> G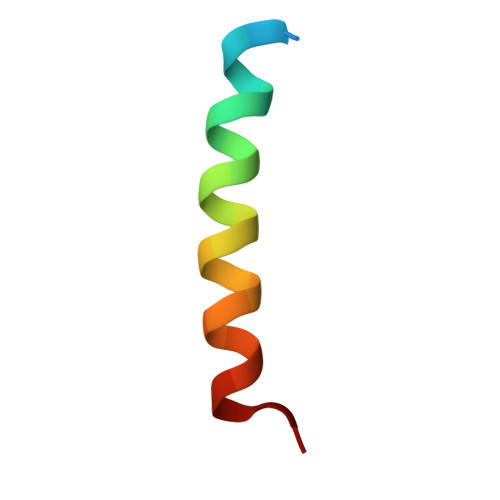SGGRPEIWYAQELRRIGDEFNAYYAR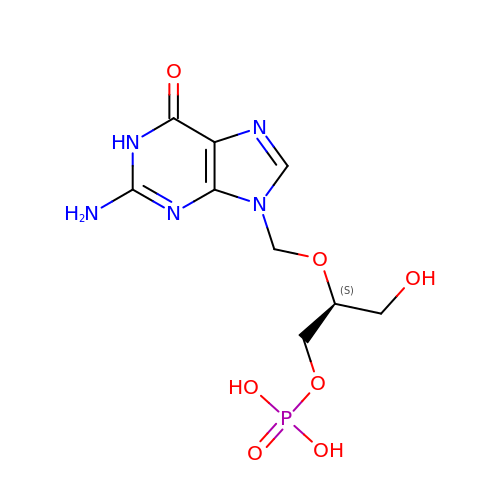N9-1-HYDROXY-PROP-2-OXYMETHYL-GUANINE-3'-MONOPHOSPHATE | C9 H14 N5 O7 P | LSJIZCGOXSEZNF-YFKPBYRVSA-N> MEGNTILKIVLICTILAGLFGQVVPVYAENTTYQTPTGIYYEVRGDTIYMINVTSGEETPIHLFGVNWFGFETPNHVVHGLWKRNWEDMLLQIKSLGFNAIRLPFCTESVKPGTQPIGIDYSKNPDLRGLDSLQIMEKIIKKAGDLGIFVLLDYHRIGCTHIEPLWYTEDFSEEDFINTWIEVAKRFGKYWNVIGADLKNEPHSVTSPPAAYTDGTGATWGMGNPATDWNLAAERIGKAILKVAPHWLIFVEGTQFTNPKTDSSYKWGYNAWWGGNLMAVKDYPVNLPKNKLVYSPHVYGPDVYNQPYFGPAKGFPDNLPDIWYHHFGYVKLELGYSVV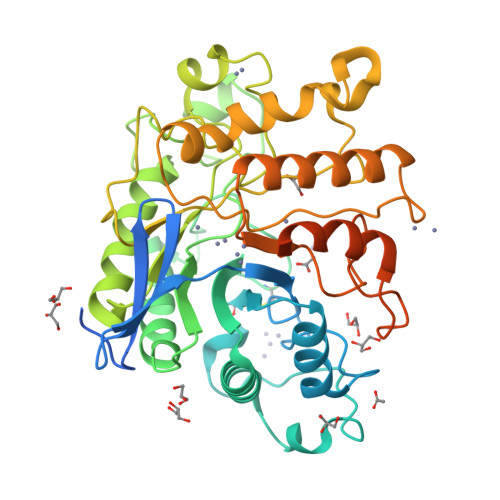IGEFGGKYGHGGDPRDVIWQNKLVDWMIENKFCDFFYWSWNPDSGDTGGILQDDWTTIWEDKYNNLKRLMDSCSKSSSSTQSVIRSTTPTKSNTSKKICGPAILIILAVFSLLLRRAPR>[4x]MAKPQVTILATGGTIAGSGESSVKSSYSAGAVTVDKLLAAVPAINDLATIKGEQISSIGSQEMTGKVWLKLAK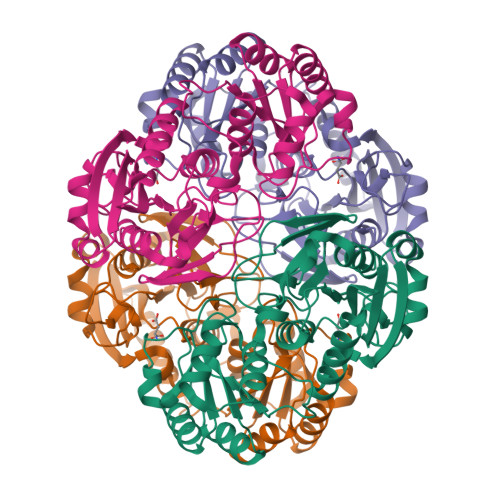RVNELLAQKETEAVIITHGTDTMEETAFFLNLTVKSQKPVVLVGAMRPGSSMSADGPMNLYNAVNVAINKASTNKGVVIVMNDEIHAAREATKLNTTAVNAFASPNTGKIGTVYYGKVEYFTQSVRPHTLASEFDISKIEELPRVDILYAHPDDTDVLVNAALQAGAKGIIHAGMGNGNPFPLTQNALEKAAKSGVVVARSSRVGSGSTTQEAEVDDKKLGFVATESLNPQKARVLLMLALTKTSDREAIQKIFSTY DITHIOBIS-(PROPANE) 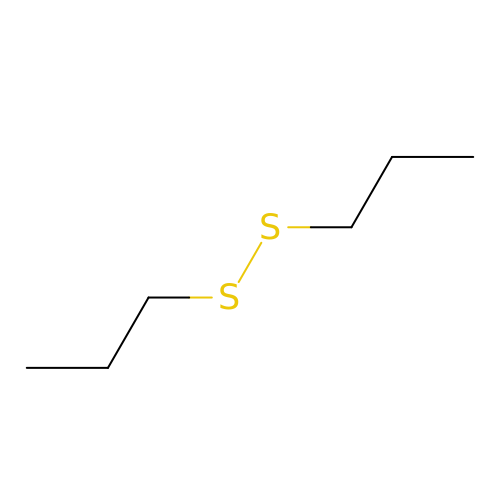| C6 H14 S2 | ALVPFGSHPUPROW-UHFFFAOYSA-N> SQAATPAADGKVKISIDPLTRVEGHLKIEVEVKDGKVVDAKCSGGMFRGFEQILRGRDPRDSSQIVQRICGVCPTAHCTASVMAQDDAFGVKVTTNGRITRNLIFGANYLQSHILHFYHLAALDYVKGPDVSPFVPRYANADLLTDRIKDGAKADATNTYGLNQYLKALEIRRICHEMVAMFGGRMPHVQGMVVGGATEIPTADKVAEYAARFKEVQKFVIEEYLPLIYTLGSVYTDLFETGIGWKNVIAFGVFPEDDDYKTFLLKPGVYIDGKDEEFDSKLVKEYVGHSFFDHSAPGGLHYSVGETNPNPDKPGAYSFVKAPRYKDKPCEVGPLARMWVQNPELSPVGQKLLKELYGIEAKKFRDLGDKAFSIMGRHVLRAEETWLTAVAVEKWLKQV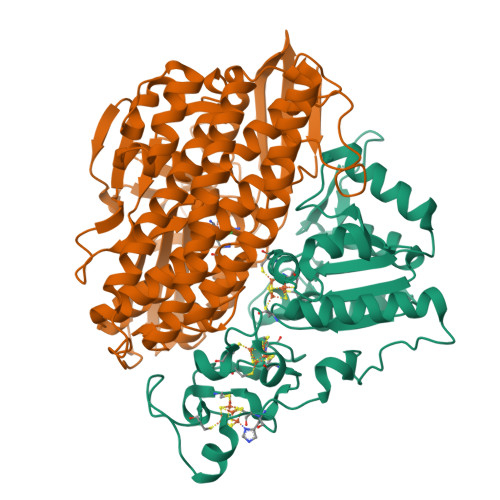QPGAETYVKSEIPDAAEGTGFTEAPRGALLHYLKIKDKKIENYQIVSATLWNANPRDDMGQRGPIEEALIGVPVPDIKNPVNVGRLVRSYDPULGCAVH;> MTEGAKKAPVIWVQGQGCTGCSVSLLNAVHPRIKEILLDVISLEFHPTVMASEGEMALAHMYEIAEKFNGNFFLLVEGAIPTAKEGRYCIVGETLDAKAHHHEVTMMELIRDLAPKSLATVAVGTCSAYGGIPAAEGNVTGSKSVRDFFADEKIEKLLVNVPGCPPHPDWMVGTLVAAWSHVLNPTEHPLPELDDDGRPLLFFGDNIHENCPYLDKYDNSEFAETFTKPGCKAELGCKGPSTYADCAKRRWNNGINWCVENAVCIGCVEPDFPDGKSPFYVAE> MADNQPVPLTPAPPGMVSLGVNENGEEEMTVIGGDGSGTGFSGNEAPIIPGSGSLQADLGKKSLTRLQAESSAAIHATAKWTTENLAKTQAAQAERAKAAMLSQQAAKAKQAKLTQHLKDVVDRALQNNKTRPTVIDLAHQNNQQMAAMAEFIGRQKAIEEARKKAEREAKRAEEAYQAALRAQEEEQRKQAEIERKLQEARKQEAAAKAKAEADRIAAEKAEAEARAKAEAERRKAEEARKALFAKAGIKDTPGCLEHHH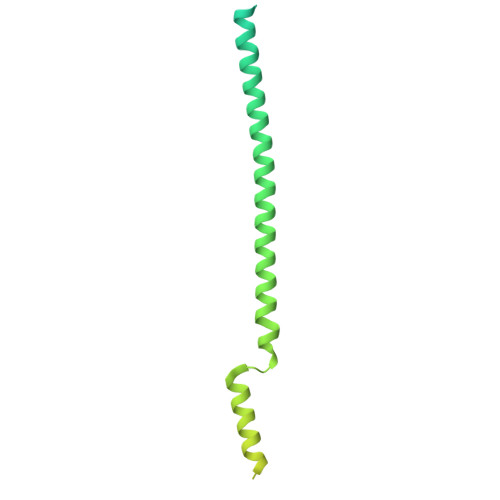HHH> PLKVEKFATANRGNGLRAVTPLRPGELLFRSDPLAYTVCKGSRGVVCDRCLLGKEKLMRCSQCRVAKYCSAKCQKKAWPDHKRECKCLKSCKPRYPPDSVRLLGRVVFKLMDGAPSESEKLYSFYDLESNINKLTEDRKEGLRQLVMTFQHFMREEIQDASQLPPAFDLFEAFAKVICNSFTICNAEMQEVGVGLYPSISLLNHSCD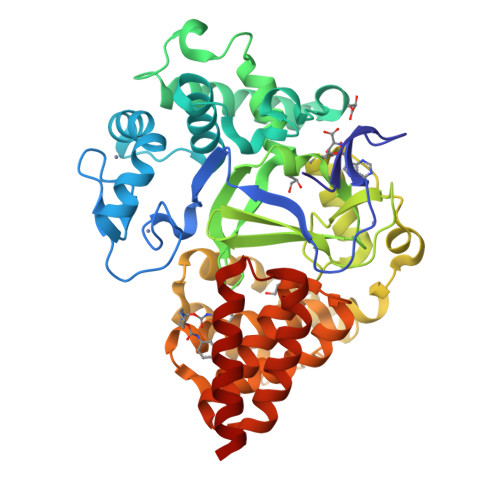PNCSIVFNGPHLLLRAVRDIEVGEELTICYLDMLMTSEERRKQLRDQYCFECDCFRCQTQDKDADMLTGDEQVWKEVQESLKKIEELKAHWKWEQVLAMCQAIISSNSERLPDINIYQLKVLDCAMDACINLGLLEEALFYGTRTMEPYRIFFPGSHPVRGVQVMKVGKLQLHQGMFPQAMKNLRLAFDIMRVTHGREHSLIEDLILLLEECDANIRA>[2x]MSIYTLGIDVGSTASKCIILKDGKEIVAKSLVAVGTGTSGPARSISEVLENAHMKKEDMAFTLATGYGRNSLEG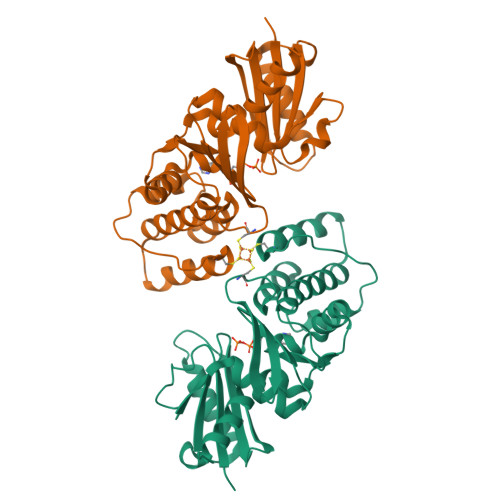IADKQMSELSCHAMGASFIWPNVHTVIDIGGQDVKVIHVENGTMTNFQMNDKCAAGTGRFLDVMANILEVKVSDLAELGAKSTKRVAISSTCTVFAESEVISQLSKGTDKIDIIAGIHRSVASRVIGLANRVGIVKDVVMTGGVAQNYGVRGALEEGLGVEIKTSPLAQYNGALGAALYAYKKAAKSAWSHPQFEK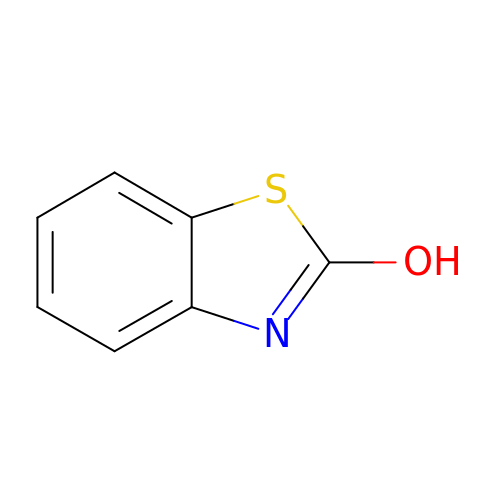1,3-benzothiazol-2-ol | C7 H5 N O S | YEDUAINPPJYDJZ-UHFFFAOYSA-N>MSRRFTVTSLPPAASAASADPESRRHSVADPRRLPREDVKGDGNPKESSPFINSTDTEKGREYDGRNMALFEEEMDTSPMVSSLLSGLANYTNLPQGSREHEEAENNEGGKKKPVQAPRMGTFMGVYLPCLQNIFGVILFLRLTWVVGIAGIMESFCMVFICCSCTMLTAISMSAIATNGVVPAGGSYYMISRSLGPEFGGAVGLCFYLGTTFAGAMYILGTIEILLAYLFPAMAIFKAEDASGEAAAMLNNMRVYGTCVLTCMATVVFVGVKYVNKFALVFLGCVILSILAIYAGVIKSAFDPPNFPICLLGNRTLSRHGFDVCAKLAWEGNETVTTRLWGLFCSSRLLNATCDEYFTRNNVTEIQGIPGAASGLIKENLWSSYLTKGVIVERRGMPSVGLADGTPVDMDHPYVFSDMTSYFTLLVGIYFPSVTGIMAGSNRS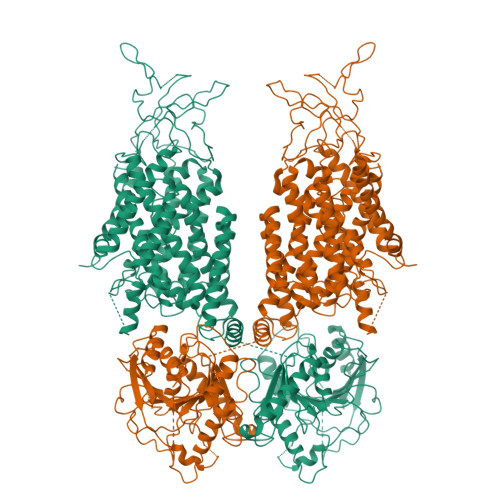GDLRDAQKSIPTGTILAIATTSAVYISSVVLFGACIEGVVLRDKFGEAVNGNLVVGTLAWPSPWVIVIGSFFSTCGAGLQSLTGAPRLLQAISRDGIVPFLQVFGHGKANGEPTWALLLTACICEIGILIASLDEVAPILSMFFLMCYMFVNLACAVQTLLRTPNWRPRFRYYHWTLSFLGMSLCLALMFICSWYYALVAMLIAGLIYKYIEYRGAEKEWGDGIRGLSLSAARYALLRLEEGPPHTKNWRPQLLVLVRVDQDQNVVHPQLLSLTSQLKAGKGLTIVGSVLEGTFLDNHPQAQRAEESIRRLMEAEKVKGFCQVVISSNLRDGVSHLIQSGGLGGLQHNTVLVGWPRNWRQKEDHQTWRNFIELVRETTAGHLALLVTKNVSMFPGNPERFSEGSIDVWWIVHDGGMLMLLPFLLRHHKVWRKCKMRIFTVAQMDDNSIQMKKDLTTFLYHLRITAEVEVVEMHESDISAYTYEKTLVMEQRSQILKQMHLTKNEREREIQSITDESRGSIRRKNPANPRLRLNVPEETACDNEEKPEEEVQLIHDQSAPSCPSSSPSPGEEPEGERETDPEVHLTWTKDKSVAEKNKGPSPVSSEGIKDFFSMKPEWENLNQSNVRRMHTAVRLNEVIVNKSRDAKLVLLNMPGPPRNRNGDENYMEFLEVLTEQLDRVMLVRGGGREVITIYS[2x]> MGSSHHHHHHSSGLVPRGSHKREAVQEERQRGKDRNENEVESTSSANEDMPVERILEAELAVEPKTETYVE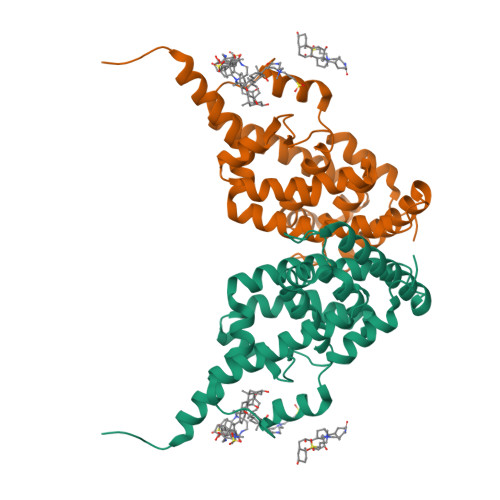ANMGLNPSSPNDPVTNICQAADKQLFTLVEWAKRIPHFSELPLDDQVILLRAGWNELLIASFSHRSIAVKDGILLATGLHVHRNSAHSAGVGAIFDRVLTELVSKMRDMQMDKTELGCLRAIVLFNPDSKGLSNPAEVEALREKVYASLEAYCKHKYPEQPGRFAKLLLRLPALRSIGLKCLEHLFFFKLIGDTPIDTFLMEMLEAPHQMT>[4x]MLKGKKAVVTGSTSGIGLAMATELAKAGADV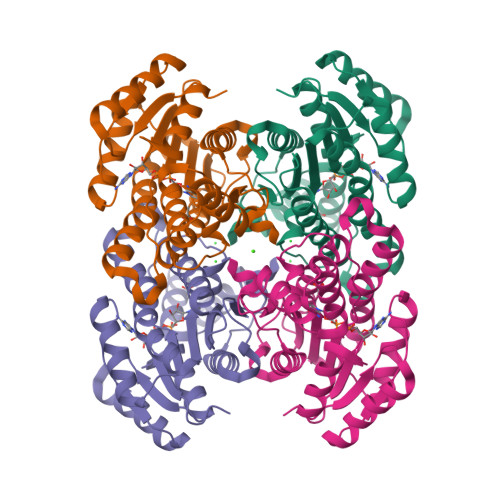VINGFGQPEDIERERSTLESKFGVKAYYLNADLSDAQATRDFIAKAAEALGGLDILVNNAGIQHTAPIEEFPVDKWNAIIALNLSAVFHGTAAALPIMQKQGWGRIINIASAHGLVASVNKSAYVAAKHGVVGLTKVTALENAGKGITCNAICPGWVRTPLVEKQIEAISQQKGIDIEAAARELLAEKQPSLQFVTPEQLGGAAVFLSSAAADQMTGTTLSLDGGWTAR>GPAGETTKLDLSVKAVGWGAADASGVLQPIKFYRRVPGERDVKIRVLYSGVCNFDMEMVRNKWGFTRYPYVFGHETAGEVVEVGSKVEKFKVGDKVAVGCMVGSCGQCYNCQSGMENYCPEPNMADGSVYREQGERSYGGCSNVMVVDEKFVLRWP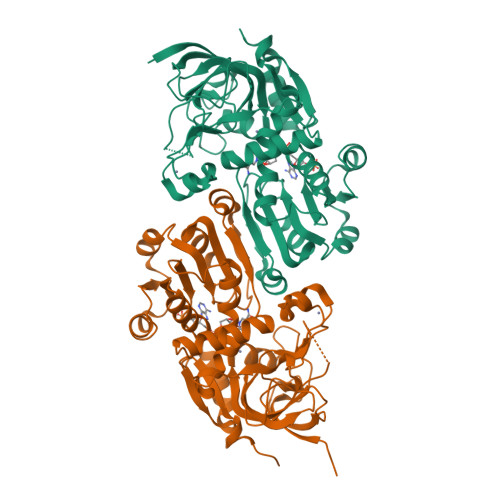ENLPQDKGVALLCAGVVVYSPMKHLGLDKPGKHIGVFGLGGLGSVAVKFIKAFGGKATVISTSRRKEKEAIEEHGADAFVVNTDSEQLKALAGTMDGVVDTTPGGRTPMSLMLNLLKFDGAVMLVGAPESLFELPAAPLIMGRKKIIGSSTGGLKEYQEMLDFAAKHNIVCDTEVIGIDYLSTAMERIKNLDVKYRFAIDIGNTLKFEE[2x]> MGHHHHHHSHMLPPEQWSHTTVRNALKDLLKDMNQSSLAKECPLSQSMISSIVNSTY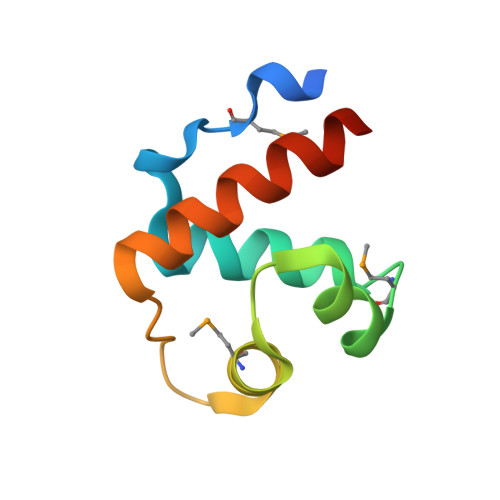YANVSAAKCQEFGRWYKHFKKTKDMM> MWRSSGVSFTRYASEMAALLRQCLKEPYRTQAMQRNQIHLKETVYQQGQVLTRETFND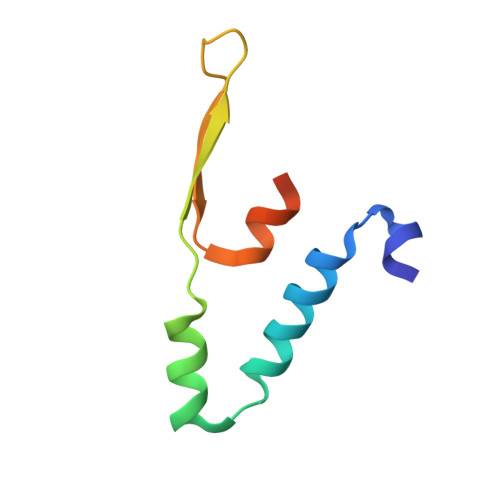IKKAFEAAAKHAGEK>GPGYQDPNSSLLEALNVRVVGSGEKVLVLAHGVGTDQSAWQRILPYFVRDHRVVLYDLVCAGSVNPDYFDFRRYTSLDAFVDDLLAILDALRLGRCTYVGHSVSASIGILASIRRPDLFAKLILIGASPRFLNDKNYHGGFADGEIDTVFAAMEANYAAWVSGFAPLAVGADVPEAVREFSRTLFNMRPDITLFVSRMVFNSDLRGVLGLVTVPCSVLQTSKDHSVPESMAAYLKENLGGRTTVHMLDIEGHLPHLSAPNLLAQELRRALPR[2x]

Strigolactones (SLs) and karrikins (KARs) are two classes of structurally related molecules that mediate signaling pathways to stimulate seed germination. SL and KAR have been reported to be recognized by the homologous proteins D14 (DWARF14)14–17 and HTL (HYPOSENSITIVE TO LIGHT; also known as KAI2, KARRIKIN INSENSITIVE2), respectively. To elucidate the structural basis of ligand specificity, we determined the crystal structures of ShHTL1, ShHTL4, ShHTL7, and ShD14 and compared their structures with those reported for ShHTL331 and ShHTL529. All the structures were highly similar to one another, consisting of a canonical α/β hydrolase domain and a helical cap.

ShD14 showed a high sequence conservation with other angiosperms D14 (e.g., sequence identity of 75% with AtD14 and OsD14) and maintained one D14 copy in Striga as in other nonparasitic plants, which strongly suggested that ShD14 had a conserved function with D14 from other angiosperms. In contrast, although only one D14 ortholog, ShD14, has been found in Striga, it showed no enzymatic activity toward Yoshimulactone Green (YLG), a fluorogenic SL agonist that becomes fluorescent when it is hydrolyzed by AtD14 or some HTL enzymes, despite possessing conserved catalytic triad residues. Here, we also demonstrated the hydrolytic activity of ShD14 toward rac-GR24 and 5DS, despite the demonstration of no hydrolytic activity toward YLG in a previous study. ShD14 was able to hydrolyze rac-GR24 and 5DS but not YLG, suggesting that ShD14 might also serve as an SL receptor. ShD14 and OsD14 have bulky residues in their pockets, such as F125ShD14/F176OsD14, W154ShD14/W205OsD14, and F194ShD14/F245OsD14 (corresponding to residues 124, 153, and 194 in ShHTLs), making their pockets smaller than those of the divergent clade. However, these differences between ShD14 and ShHTL7 did not seem to influence their hydrolytic activity toward rac-GR24. In contrast, the corresponding residue of L142 in the D14 group was the highly conserved V143ShD14, which avoids such steric hindrance. A rac-GR24-dependent ShD14–ShMAX2 interaction was also observed, which strongly suggested that ShD14 might serve as an SL receptor. Consistent with the results of the Y2H assays, a direct interaction was detected between ShMAX2 and ShD14 in a rac-GR24-dependent manner, as in the AtD14–AtMAX2 interaction. Moreover, the transcripts of ShD14 remained unchanged during the conditioning and germination process of Striga seeds;28 therefore, it was likely that ShD14 did not function in germination.>GHMKLCTFTITQKEFMNQHWYHCHTCKMVDGVGVCTVCAKVCHKDHEISYAKYGSFFCDCGAKEDGSCLALVK[3x]

The N-end rule pathway is a proteolytic system involving the destabilization of N-terminal amino acids, known as N-degrons, which are recognized by N-recognins. The E3 ligases of the UBR subfamily recognize and degrade N-degrons through the ubiquitin-proteasome system. However, unlike other UBR proteins, UBR4, despite having only the UBR box domain, can recognize both type-1 and type-2 N-degron. Our findings suggest that the UBR box of UBR4 recognizes type-1 N-terminal arginine and type-2 N-terminal amino acids containing an aromatic ring, such as tyrosine, tryptophan, and phenylalanine through pi-interaction with two phenylalanines of the UBR box of UBR4.

First, we determined the ligand-free structure of UBR4UBR. The structure of UBR4UBR, like other UBR boxes, is composed of three α-helices and two antiparallel β-sheets. The UBR4UBR coordinates three zinc ions. One zinc ion (Zn1) is canonically coordinated by two cysteines and two histidines similar to the other UBR boxes. However, whereas two zinc ions (Zn2 and Zn3) were coordinated by six cysteines and one histidine in the structure of the UBR boxes of UBR1 and UBR2, two zinc ions were coordinated by seven cysteines in UBR4UBR. Besides differences in the residues coordinating zinc, there was also a structural difference between UBR4UBR and the UBR boxes of UBR1 and UBR2. The carboxyl group of Asp1715 and the oxygen atom between Phe1713 were conserved at the same positions in the structure of UBR4UBR as in the UBR box of UBR2. However, in the structure of UBR4UBR, there is a unique feature where the aspartic acid residue (Asp1721), which is one of the main features of N-recognins such as UBR1 and UBR2, is located far away from the ligand-binding site. In other words, in UBR4UBR, Asp1721 may not be involved in ligand-binding unlike other the UBR boxes of UBR1 and UBR2. First, as observed in other N-recognin structures, during crystallization of UBR4UBR the amino acid at the N-terminus was bound to the ligand-binding site of other UBR4UBR molecules in the apo UBR4UBR structure.> GPLGSPEFIILQTYRAIADYEKTSGSEMALSTGDVVEVVEKSESGWWFCQMKAKRGWIPASFLEPLDSPDETEDPEPNYAGEPYVAIKAYTAV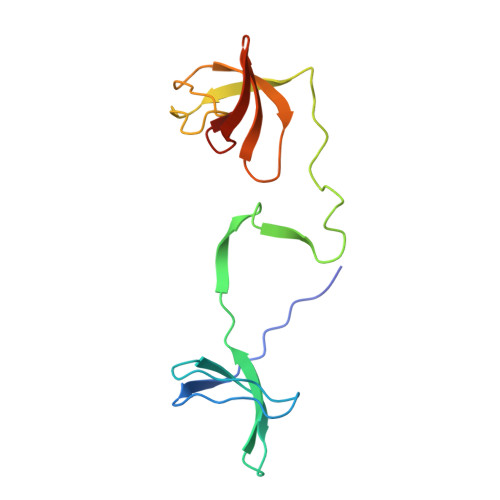EGDEVSLLEGEAVEVIHKLLDGWWVIRKDDVTGYFPSMYLQKSGQ> CGCXAAUUAGC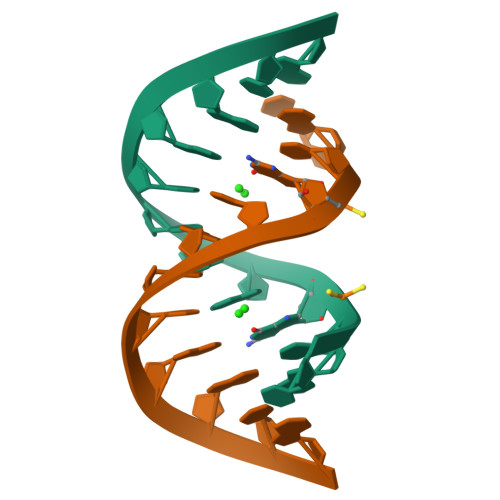G> GMETTHYSIAQHFSSGDFPAVYACFNDIIEWNIIGNQVVKGKADVIDF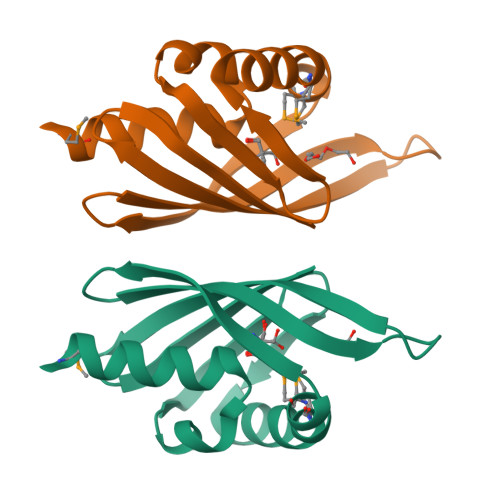CNKMLPEMKGAVLTNDNVIQNENQIVIEGKCRYFDAEGKEAFVSYCDIYRFENDTIKTITSYCI> EYDYLFKVVLIGDSGVGKSNLLSRFTRNEFNLES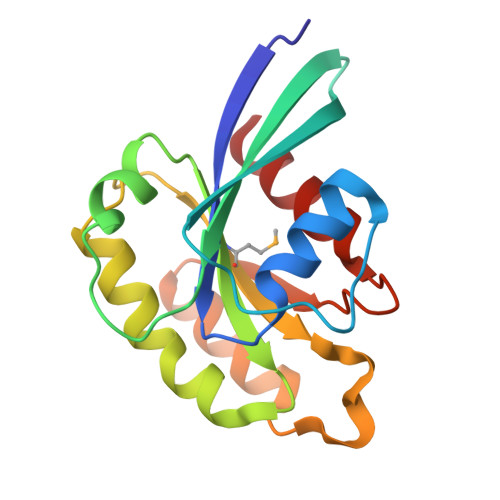KSTIGVEFATRSIQVDGKTIKAQIWDTAGLERYRAITSAYYRGAVGALLVYDIAKHLTYENVERWLKELRDHADSNIVIMLVGNKSDLRHLRAVPTDEARAFAEKNGLSFIETSALDSTNVEAAFQTILTEIY>[2x]MIAEAWSPATDERLRAAGIDAEDARRVVVTALEEDLRYGADVTSDATVPADAVTEAVVASRQPGVLAGLPVALAVLDLVTGGRFEVAECRADGDRLGPGDVALRVTAATRELLVAERTMLNLLCHLSGVATLTARWNDALAGTHCKVRD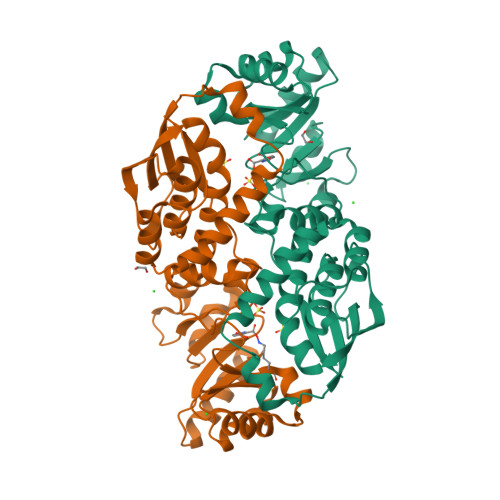SRKTLPGLRLLEKYAVRRGGGQNHRLGLGDAILIKDNHIVAGGSAGAALQAARAHTPGLPCEVEVTTLAELDEVLALGADEVMLDNFTVEQCVEAVRRRDAARTRTRLEASGGLTLDVAAAYARTGVDLLAVGALTHSAPALDLGLDFAPRTEGDVRQR> TIAPITGTIKRRVI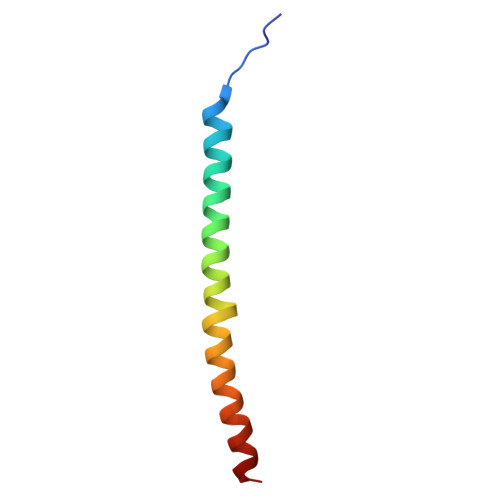MDIVLGFSLGGVMASYWWWGFHMDKINKREKFYAELAERKK> SSQIRQNYSTEVEA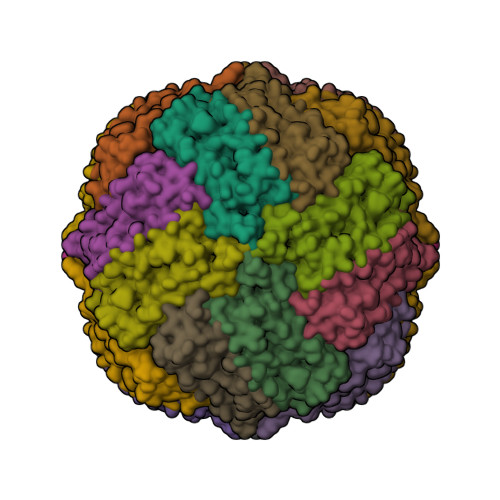AVNRLVNLYLRASYTYLSLGFYFDRDDVALEGVCHFFCELAEEKREGAERLLKMQNQRGGRALFQDLQKPSQDEWGTTLDAMKAAIVLEKSLNQALLDLHALGSAQADPHLCDFLESHFLDEEVKLIKKMGDHLTNIQRLVGSQAGLGEYLFERLTLKHD> MVPISPIETVPVKLKPGMDGPKVKQWPLTEEKIKALVEICTEMEKEGKISKIGPENPYNTPVFAIKKKDSTKWRKLVDFRELNKRTQDFWEVQLGIPHPAGIKKNKSVTVLDVGDAYFSVPLDEDFRKYTAFTIPSINNETPGIRYQYNVLPQGWKGSPAIFQSSMTKILEPFAAQNPDIVIYQYMDDLYVGSDLEIGQHRTKIEELRQHLLRWGLTTPDKKHQKEPPFLWMGYELHPDKWTVQPIVLPEKDSWTVNDIQKLVGKLNWASQIYPGIKVRQLSKLLRGTKALTEVIPLTEEAELELAENREILKEPVHGVYYDPSKDLIAEIQKQGQGQWTYQIYQEPFKNLKTGKYARMRGAHTNDVKQLTEAVQKITTESIVIWGKTPKFKLPIQKETWETWWTEYWQATWIPEWEFVNTPPLVKLWYQLEKEPIVGAETFYVDGAANRETKLGKAGYVTNKGRQKVVPLTNTTNQKTELQAIYLALQDSGLEVNIVTDSQYALGIIQAQPDKSESELVNQIIEQLIKKEKVYLAWVPAHKGIGGNEQVDKLVSAG;> PISPIETVPVKLKPGMDGPKVKQWPLTEEKIKALVEICTEMEKEGKISKIGPENPYNTPVFAIKKKDSTKWRKLVDFRELNKRTQDFWEVQLGIPHPAGLKKKKSVTVLDVGDAYFSVPLDEDFRKYTAFTIPSINNETPGIRYQYNVLPQGWKGSPAIFQSSMTKILEPFKKQNPDIVIYQYMDDLYVGSDLEIGQHRTKIEELRQHLLRWGLTTPDKKHQKEPPFLWMGYELHPDKWTVQPIVLPEKDSWTVNDIQKLVGKLNWASQIYPGIKVRQLSKLLRGTKALTEVIPLTEEAELELAENREILKEPVHGVYYDPSKDLIAEIQKQGQGQWTYQIYQEPFKNLKTGKYARMRGAHTNDVKQLTEAVQKITTESIVIWGKT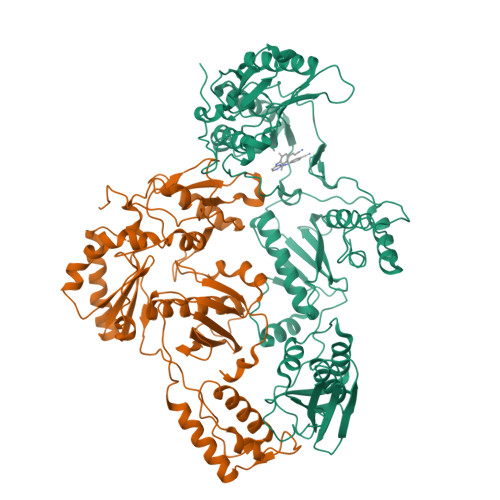PKFKLPIQKETWETWWTEYWQATWIPEWEFVNTPPLVKLWYQ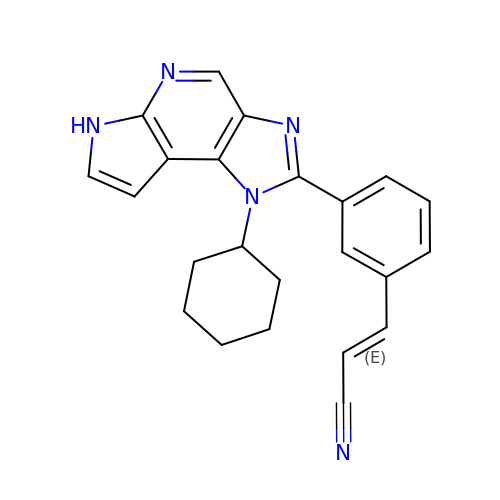(~{E})-3-[3-(3-cyclohexyl-3,5,8,10-tetrazatricyclo[7.3.0.0^{2,6}]dodeca-1(9),2(6),4,7,11-pentaen-4-yl)phenyl]prop-2-enenitrile | C23 H21 N5 | JIDRJSPIWPPOBL-FNORWQNLSA-N>[4x]TRQFLIYNEDHKRCVDAVSPSAVQTAACNQDAESQKFRWVSESQIMSVAFKLCLGVPSKTDWVAITLYACDSKSEFQKWECKNDTLLGIKGEDLFFNYGNRQEKNIMLYKGSGLWSRWKIYGTTDNLCSRGYEAMYTLLGNANGATCAFPFKFENKWYADCTSAGRSDGWLWCGTTTDYDTDKLFGYCPLKFEGSESLWNKDPLTSVSYQINSKSALTWHQARKSCQQQNAELLSITEIHEQTYLTGLTSSLTSGLWIGLNSLSFNSGWQWSDRS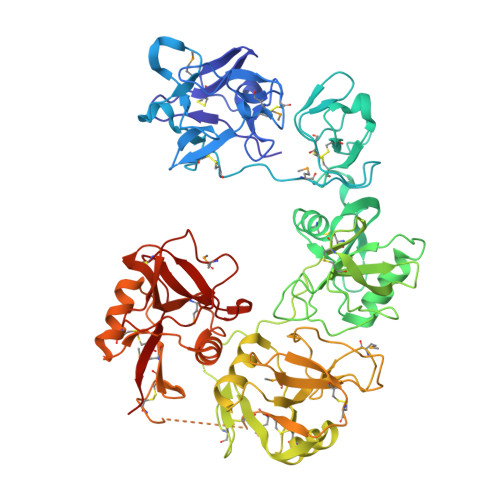PFRYLNWLPGSPSAEPGKSCVSLNPGKNAKWENLECVQKLGYICKKGNTTLNSFVIPSESDVPTHCPSQWWPYAGHCYKIHRDEKKIQRDALTTCRKEGGDLTSIHTIEELDFIISQLGYEPNDELWIGLNDIKIQMYFEWSDGTPVTFTKWLRGEPSHENNRQEDCVVMKGKDGYWADRGCEWPLGYICKMKSRSQGPEIVEVEKGCRKGWKKHHFYCYMIGHTLSTFAEANQTCNNENAYLTTIEDRYEQAFLTSFVGLRPEKYFWTGLSDIQTKGTFQWTIEEEVRFTHWNSDMPGRKPGCVAMRTGIAGGLWDVLKCDEKAKFVCKHWAHHHHHH>SLFELGKMILQETGKNPAKSYGVYGCNCGVGGRGKPKDATDRCCYVHKCCYKKLTGCDPKKDRYSYSWKDKTIVCGENNSCLKELCECDKAVAICLRENLD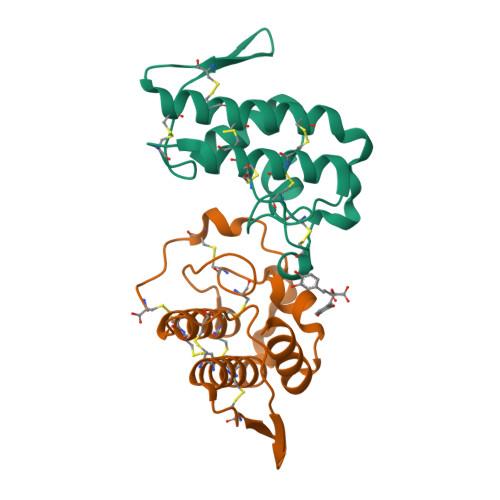TYNKKYRYNYLKPFCKKADPC[2x]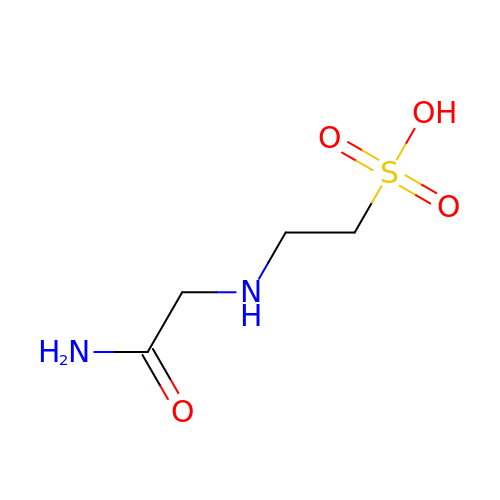N-(2-acetamido)-2-aminoethanesulfonic acid | C4 H10 N2 O4 S | DBXNUXBLKRLWFA-UHFFFAOYSA-N> MSQIIWGAYAQRNTEDHPPAYAPGYKTSVLRSPKNALISIAETLSEVTAPHFSADKFGPKDNDLILNYAKDGLPIGERVIVHGYVRD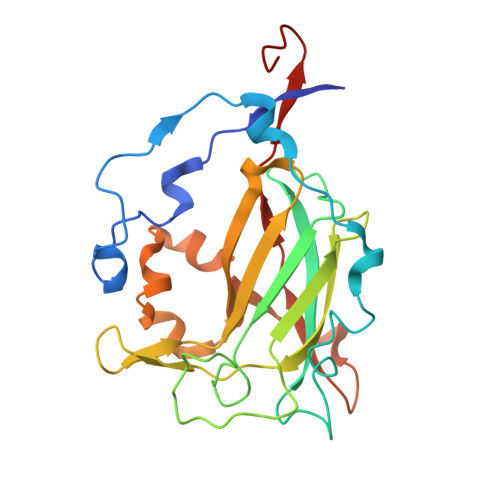QFGRPVKNALVEVWQANASGRYRHPNDQYIGAMDPNFGGCGRMLTDDNGYYVFRTIKPGPYPWRNRINEWSPAHIHFSLIADGWAQRLISQFYFEGDTLIDSCPILKTIPSEQQRRALIALEDKSNFIEADSRCYRFDITLRGRRATYFENDLT> KGHLTRLGLEFFDQPAVPLARAFLGQVLVRRLPNGTELRGRIVETEAYLGPEDEAAHSRGGRQTPRNRGMFMKPGTLYVYIIYGMYFCMNISSQGDGACVLLRALEPLEGLETMRQLRSTLRKGTASRVLKDRELCSGPSKLCQALA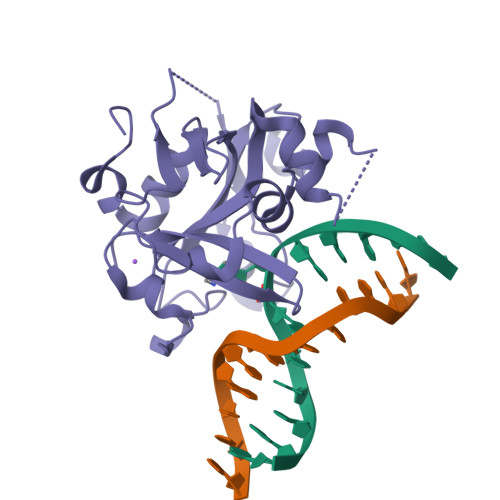INKSFDQRDLAQDEAVWLERGPLEPSEPAVVAAARVGVGHAGEWARKPLRFYVRGSPWVSVVDRVAEQDTQA>[2x]SARVGSQNGVQMLSPSEIPQRDWFPSDFTFGAATSAYQIEGAWNEDGKGESNWDHFCHNHPERILDGSNSDIGANSYHMYKTDVRLLKEMGMDAYRFSISWPRILPKGTKEGGINPDGIKYYRNLINLLLENGIEPYVTIFHWDVPQALEEKYGGFLDKSHKSIVEDYTYFAKVCFDNFGDKVKNWLTFNDPQTFTSVSYGTGVFAPGRCSPGLDCAYPTGNSLVEPYTAGHNILLAHAEAVDLYNKHYKRDDTRIGLAFDVMGRVPYGTSFLDKQAEERSWDINLGWFLEPVVRGDYPFSMRSLARERLPFFKDEQKEKLAGSYNMLGLNYYTSRFSKNIDISPNYSPVLNTDDAYASQEVNGPDGKPIGPPMGNPWIYMYPEGLKDLLMIMKNKYGNPPIYITENGIGDVDTKETPLPMEAALNDYKRLD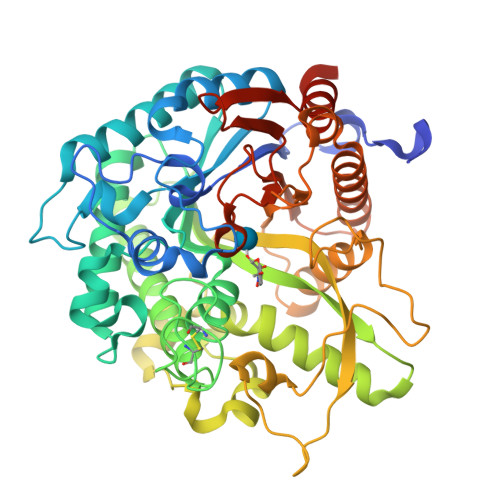YIQRHIATLKESIDLGSNVQGYFAWSLLDNFEWFAGFTERYGIVYVDRNNNCTRYMKESAKWLKEFNTAKKPSKKILTPA>SDPVDYQAEDATIVQGAVESNHAGYTGTGFVNYDNVAGSSVEWTVTVPSAGTYDVVVRYANGTTTSRPLDFSVNGSISASGVAFGSTGTWPAWTTKTVRVTLAAGVNKIKAVATTANGGPNV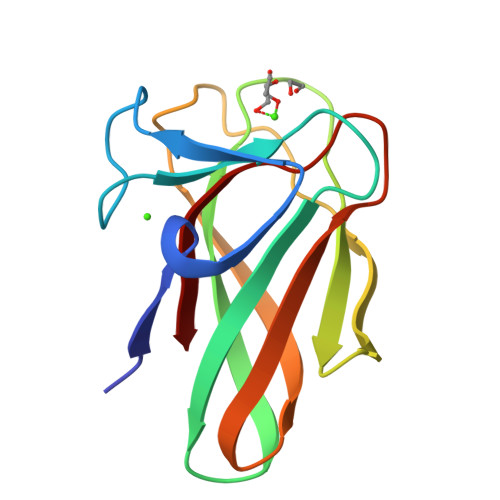DKITL[2x]>[2x]MGSPTDNYIYAVCSPAKFSPSSGYETNLNSLLSSFVTSTAQTRYANFTVPTGKPEPTVTV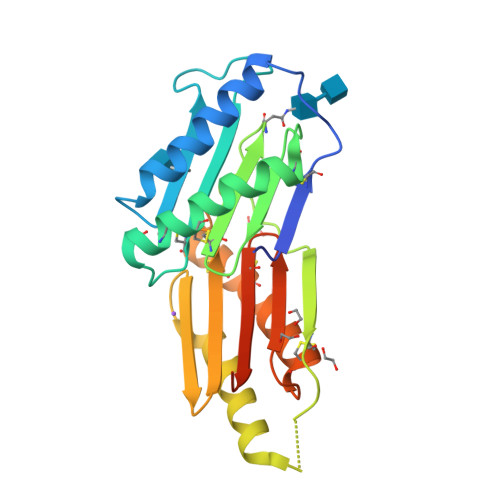YGIYQCRGDLDPTACSTCVSSAVAQVGALCSNSYSGFLQMENCLIRYDNKSFLGVQDKTLILNKCGQPMEFNDQDALTKASDVIGSLGTGDGSYRTGGNGNVQGVAQCSGDLSTSQCQDCLSDAIGRLKSDCGMAQGGYVYLSKCYARFSVGGSHARQLEGSENLYFQ N-{3-[(4S)-2-amino-5,5-difluoro-4-(fluoromethyl)-5,6-dihydro-4H-1,3-oxazin-4-yl]-4-fluorophenyl}-5-cyanopyridine-2-carboxamide 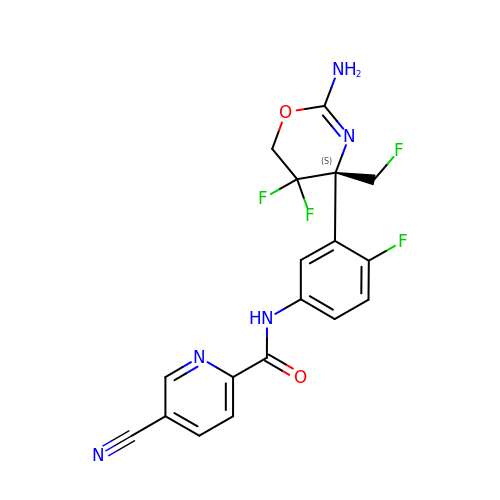| C18 H13 F4 N5 O2 | OIFTUNMTFHXWBX-QGZVFWFLSA-N> MRRLAFLVVAFCLAVGCFFSPVSKAEGVMSGGDGDKVAVGKDGMVATAHPLASKIGAEVLKKGGNAIDAAIAIQYALNVTEPMMSGIGGGGFMMVYDGETRETSIINSRERAPEGAKPDMFLDEDGKVIPFSERSRHGNAVGVPGTLKGLEAAHKKWGTKKMEDLISPSIKLTEEGFPIDSVLADAIKDHQDKLSKTAAKDIFLPDGEPLKEGDILVQKDLAKTFKLIRKEGSKAFYDGEIGRAIADVVQDFGGSMTPDDLSRYEVTTDKPIWGEYHGYDIASMPPPSSGGVFMLQVLKLIDDFHLSQYDPKSFEKYHLLAETMHLSYADRAAYAGDPEFVDVPLRGLLDPDYIKERQKLISLDSMNRDVKEGDPWKYEEGEPNYEI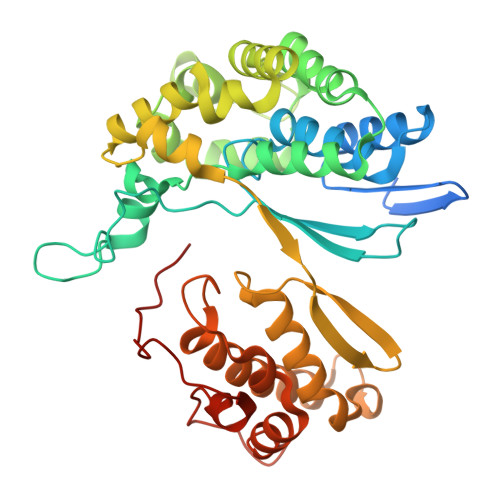VPQPEDKTIGE>[4x]AAUUGAAAAAUCAAUAGAUUUAAACCUAGUGAAGAGCAUUUGAACAAUGUGCUAGGGUAGUAUGGGAUAAGUCGAUAACUAAAAUGAAUUGGGAUACUGAUUGAUUUUAGUGGUGGAUUUUACAGCAAUGUAAAAAGGACUAAUAGUAAAAGCUAUUAAUCGCAAAGUACUACGUGGAAUUUGUGCAGGUGUAAGGUACGAAACUUUCGAGUGUGACAAUAGACGCUCCAGUGGAGAAUAAUCUAAGUUAGGUGGA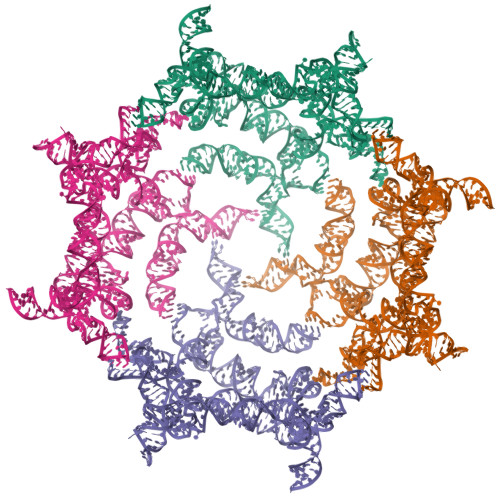AGUGUGAGAAGCUUGGCAGACCUUAGAAAACUCAAACCAAGCGCUUUGCAGAGAAACUGAGAAAUCAGUGUUUAACGAAAGAAGUCGGUACGAGUAGCUUAAUGCAGCAAUUUAUUUACAGAUGACAAAUAAUAAAAAUGGGACUCUUAUGUAAAUGCUGAAUGUUCAAGUGAAAGUUAUUAGCCAGUAGAGCUAGAUCAUACAGAAAAAGCAAAGAGAAGCUAUUGGGUAGCGCCCGAUAGUUCAGCCUCUUUGGGUAUGUGACUGAAUAACACUGUAAACAAAGGAAGCAGGAAGAAAAGCCUAAAUCUGUUGAUUUUUGAG>[4x]SMRPSLKTLQEKGLIKDQIFGSHLHKVCERENSTVPWFVKQCIEAVEKRGLDVDGIYR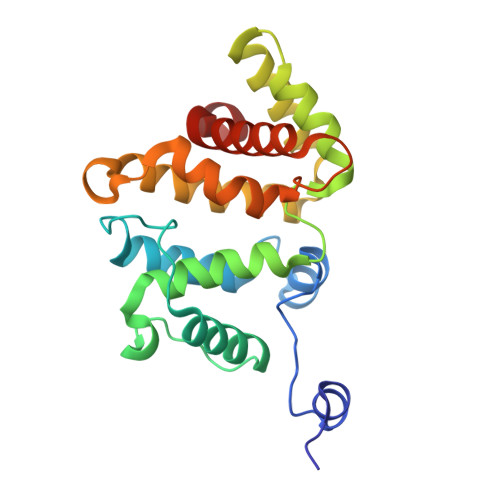VSGNLATIQKLRFIVNQEEKLNLDDSQWEDIHVVTGALKMFFRELPEPLFPYSFFEQFVEAIKKQDNNTRIEAVKSLVQKLPPPNRDTMKVLFGHLTKIVAKASKNLMSTQSLGIVFGPTLLRAENETGNMAIHMVYQNQIAELMLSEYSKIFGSE>MAEIKHYQFNVVMTCSGCSGAVNKVLTKLEPDVSKIDISLEKQLVDVYTTLPYDFI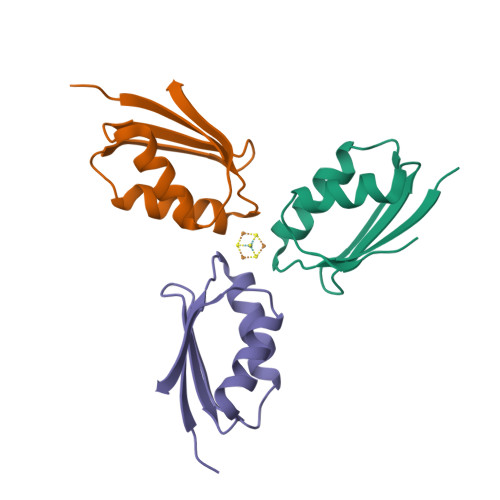LEKIKKTGKEVRSGKQL[12x]The enzyme responsible for the core function of heterotrophic nitrification is pyruvic oxime dioxygenase (POD). POD is a non-heme, Fe(II)-dependent enzyme that catalyzes the dioxygenation of pyruvic oxime to produce pyruvate and nitrite. Bacteria of the genera Alcaligenes and Pseudomonas are known to perform heterotrophic nitrification, which produces nitrite from ammonia using pyruvate oxime (PO) as an intermediate metabolite. PODs have additional sequences at the N-terminus consisting of 20–30 amino acid residues that are not present in class II aldolases, corresponding to the disordered region of AfPOD in its crystal structure.

Here, we report the first X-ray crystal structure of a novel dioxygenase, AfPOD, at 1.76 Å resolution. The final structure model of the AfPOD tetramer contains 920 amino acid residues, 693 water molecules, and 4 iron ions. The N-terminal region (Met1-Arg28) and the C-terminal region (Lys259-Arg261) of each subunit showed no apparent electron density. AfPOD has a tetrameric structure with approximate dimensions of 60 × 40 × 80 Å3. The anomalous difference Fourier maps revealed that the metal ion coordinated by three His residues was confirmed to be an iron ion, as expected from a previous biochemical analysis. In subunit A, the iron ion is located at a depth of about 8 Å at the bottom of an active site pocket with an opening of about 16 Å long and 8 Å wide at the boundary to the adjacent subunit B. Imidazole nitrogen atoms of His119, His121, and His183 and oxygen atoms of three water molecules (W1, W2, and W3) coordinate the iron ion, forming an octahedral arrangement. The α1-β1 loop (Glu45-Ala51), which is highly conserved among PODs, is also located near the iron center and is fixed by hydrogen bonding between the main-chain carbonyl oxygen of Ala51 and the iron-coordinated water 2 at distances of 2.5  Å. A 14 Å-long tunnel with a 3.5 Å diameter opening at the central cavity extends along the interface between the subunit molecules to the iron center. Notably, the α1-β1 loop (Glu45-Ala51) forms part of the tunnel in subunits B and D. However, the tunnel is blocked by a conformational change of the Glu47 in subunits A and C, which probably prevents the passage of oxygen molecules.

>[4x]MDTPLRDKSYFDERATKEMATHLQQVQRDTRETMAFACRILAMTEQEAGLAGQISVRSERPGAYWTLRFGLGFDEATPEDFIEVDRDLNTLSGEGMANPATRFHLWVYEARPDVNSIIHTHSPWATVLATARQPLVISQMDMTPLHNDCAFLGEWPGVPIADQEGVIISKALGDKRAIILAHHGYLTAGKSCQEATYLSVYLERAARLQVRAQAAFGPLTPVDDTLAAEAHDYLLKPSIVNATFDYWSRQTQGIAPLTKTR> AVSKVYARSVYDSRGNPTVEVELTTEKGVFRSIVPSGASTGVHEALEMRDGDKSKWMGKGVLHAVKNVNDVIAPAFVKANIDVKDQKAVDDFLISLDGTANKSKLGANAIL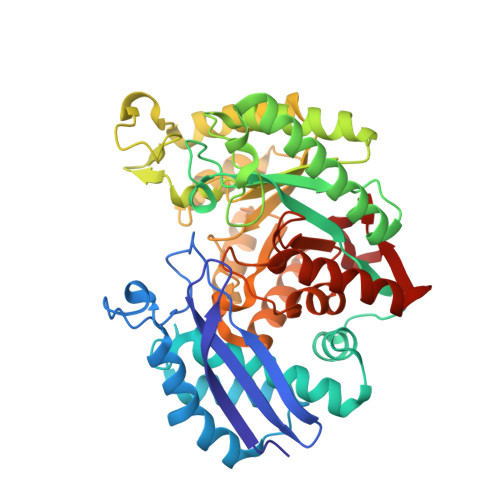GVSLAASRAAAAEKNVPLYKHLADLSKSKTSPYVLPVPFLNVLNGGSHAGGALALQEFMIAPTGAKTFAEALRIGSEVYHNLKSLTKKRYGASAGNVGDEGGVAPNIQTAEEALDLIVDAIKAAGHDGKVKIGLDCASSEFFKDGKYDLDFKNPNSDKSKWLTGPQLADLYHSLMKRYPIVSIEDPFAEDDWEAWSHFFKTAGIQIVADDLTVTNPKRIATAIEKKAADALLLAVNQIGTLSESIKAAQDSFAAGWGVMVSHRSGETEDTFIADLVVGLRTGQIKTGAPARSERLAKLNQLLRIEEELGDNAVFAGENFHHGDKL> MRSQVTLRDLFDRAVVLSHYIHNLSSEMFSEFDKRYTHGRGFITKAINSCHTSSLATPEDKEQAQQMNQKDFLSLIVSILRSWNEPLYHLVTEVRGMQEAPEAILSKAVEIEEQTKRLLERMELIVSQVHPETKENEIYPVWSGLPSLQMADEESRLSAYYNLLHCLRRDS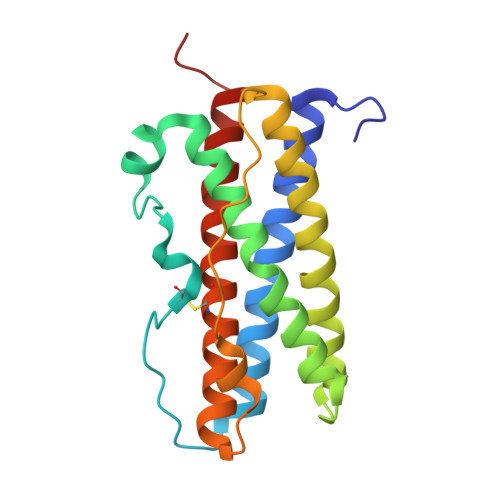HKIDNYLKLLKCRIIHNNNC> MPHVENASETYIPGRLDGKVALVTGSGRGIGAAVAVHLGRLGAKVVVNYANSTKDAEKVVSEIKALGSDAIAIKADIRQVPEIVKLFDQAVAHFGHLDIAVSNSGVVSFGHLKDVTEEEFDRVFSLNTRGQFFVAREAYRHLTEGGRIVLTSSNTSK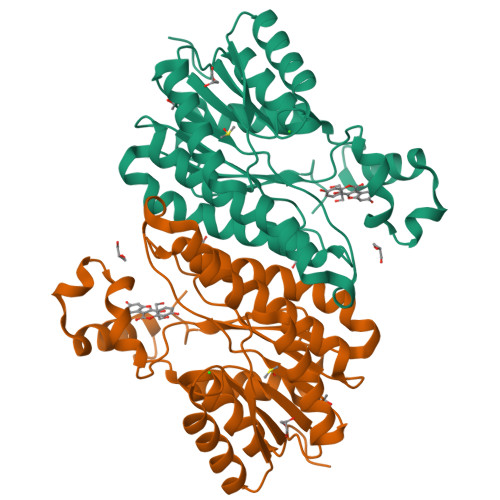DFSVPKHSLYSGSKGAVDSFVRIFSKDCGDKKITVNAVAPGGTVTDMFHEVSHHYIPNGTSYTAEQRQQMAAHASPLHRNGWPQDVANVVGFLVSKEGEWVNGKVLTLDGGAA> MFGMGFSEILVIALVAILFLGPDKLPEAMVQIAKFFNSVRKTINEAKSTFEEELHLKELKEEALSYRQSLSEVGSDISGFKNAISNHTDELQEAIEIARSGMPTDRLNESVDDLLEEDEPTGETSQRPGVT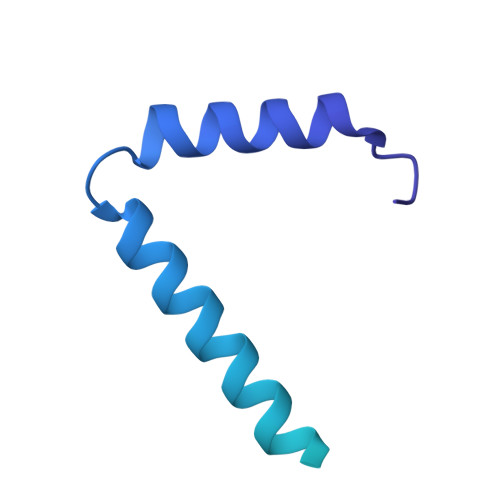EYKEMARKALEEAENSAEAQTAETPSVEDKGPESSPKESSRPAGFKHLDNEANAWSHPQFEK>[2x]MGVVLARGAFRERSMLTLPDFPLPDARGRFGPYGGRYV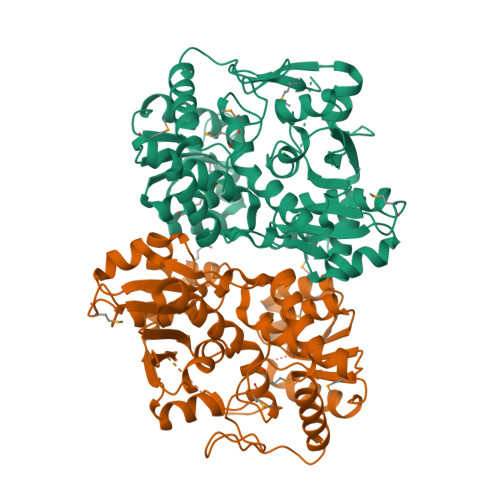PETLIPALEELEAAYREAKKDPAFLEELDHYLRQFAGRPTPLYHAKRLSEYWGGAQVFLKREDLLHTGAHKINNTLGQALLARRMGKRRVIAETGAGQHGVSVATVAALFGLECVVYMGEEDVRRQALNVFRMKLLGAEVRPVAAGSRTLKDATNEAIRDWITNVRTTFYILGSVVGPHPYPMMVRDFQSVIGEEVKRQSLELFGRLPDALIAAVGGGSNAIGLFAPFAYLPEGRPKLIGVEAAGEGLSTGRHAASIGAGKRGVLHGSYMYLLYDHDGQITPAHSVSAGLDYPGVGPEHSYYADAGVAEYASVTDEEALEGFKLLARLEGIIPALESAHAIAYAAKVVPEMDKDQVVVINLSGRGDKDVTEVMRLLGGEL> MKTQVAIIGAGPSGLLLGQLLHKAGIDNVILERQTPDYVLGRIRAGVLEQGMVDLLREAGVDRRMARDGLVHEGVEIAFAGQRRRIDLKRLSGGKTVTVYGQTEVTRDLMEAREACGATTVYQAAEVRLHDLQGERPYVTFERDGERLRLDCDYIAGCDGFHGISRQSIPAERLKVFERVYPFGWLGLLADTPPVSHELIYANHPRGFALCSQRSATRSRYFVQVPLSEKVEDWSDERFWTELKARLPSEVAEKLVTGPSLEKSIAPLRSFVVEPMQHGRLFLAGDAAHIVPPTGAKGLNLAASDVSTLYRLLLKAYREGRGELLERYSAICLRRIWKAERFSWWMTSVLHRFPDTDAFSQRIQQTELEYYLGSEAGLATI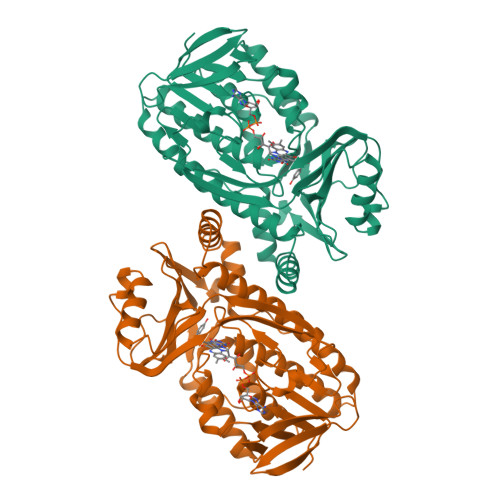AENYVGLPYEEIE> MYHRGYGGHYRGGRGGGRGHSHWHNNAPMERGGHMPSNNEGAAISSGSTGFSPLMDFFHSVEGRNYGELRSLTNETYQISENVRCTFLSIQSDPFAPGSQVRLVCPCTFSLEKVLQTTDLAAANPCRRVAAEDFILRSFHAGYRNGIPRRTSGAVQVLRPSQHVLERSTVGLVKAHQQKSGMQAEIEIFARVKLPGHGRRIDGHGAIDIFYNELVPLLEQCVVGLNEEDLHQHVICVHDQEELRSN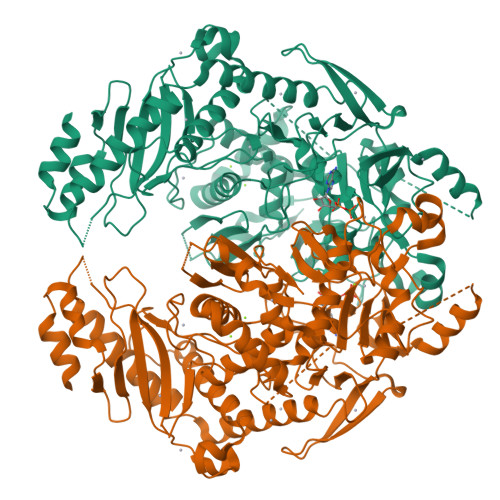LLGAGYVAFVANGAILPRDAGNSDKPLRDNAVPFQSPKSLECSFTLPHSGKTITGMGLPPGLTLIAGGGFHGKSTLLRALEVGIYNHVPDDGRTYVVVDPTAVKIRAEDRRSVHGVDISPFINNLPFGKTTNFFVTADASGSTSQAANIMEALELGSQLLLLDEDTCATNLMYRDALMQMLVPRAQEPITPFVERVADLSQNHGVSSIMVIGGSGQYFPQARVVLVMNAYQISDCTKEAKEIASNSSLPALNPPGDTASVFIPDVNRCFDPDGSFTTVRRRRGREGTKVSGIGTESIRFSEETIDLSMVEQIVEEGQVNAIAQCLALLYDGEPRIVPEMTTKGGALTQLPSPGGVCEIQRGKFNSNFSSMIAGCCSHQHDKRLELRTPSCYLPRGFTSATRHIEIGAALNRLRTLRTVTAKR>[60x]MSTFLDSFEEWYETAAASWRNLKAGAPQPKPNQQSQSVSPDREPERKDNNRGFVLPGYKYLGPGNGLDKGPPVNKADSVALEHDKAYDQQLKAGDNPYIKFNHADQDFIDSLQDDQSF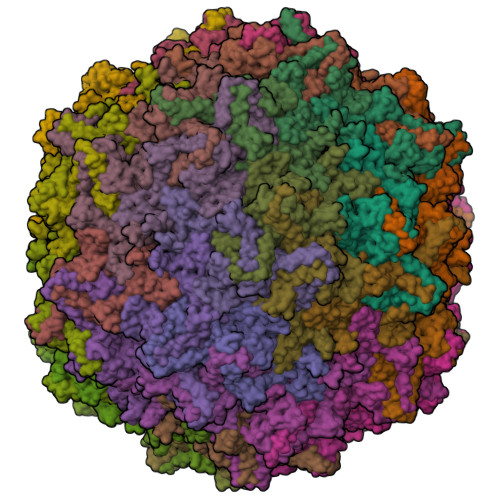GGNLGKAVFQAKKRILEPFGLVEDPVNTAPAKKNTGKLTDHYPVVKKPKLTEEVSAGGGSSAVQDGGATAEGTEPVAASEMAEGGGGAMGDSSGGADGVGNASGNWHCDSQWMGNTVITKTTRTWVLPSYNNHIYKAITSGTSQDANVQYAGYSTPWGYFDFNRFHCHFSPRDWQRLINNHWGIRPKSLKFKIFNVQVKEVTTQDQTKTIANNLTSTIQVFTDDEHQLPYVLGSATEGTMPPFPSDVYALPQYGYCTMHTNQNGARFNDRSAFYCLEYFPSQMLRTGNNFEFTFDFEEVPFHSMFAHSQDLDRLMNPLVDQYLWNFNEVDSSRNAQFKKAVKGAYGTMGRNWLPGPKFLDQRVRAYTGGTDNYANWNIWSNGNKVNLKDRQYLLQPGPVSATYTEGEASSLPAQNILGIAKDPYRSGSTTAGISDIMVTEEQEVAPTNGVGWKPYGRTVTNEQNTTTAPTSSDLDVLGALPGMVWQNRDIYLQGPIWAKIPKTDGKFHPSPNLGGFGLHNPPPQVFIKNTPVPADPPVEYVHQKWNSYITQYSTGQCTVEMVWELRKENSKRWNPEIQFTSNFSNRTSIMFAPNETGGYVEDRLIGTRYLTQNL methyl 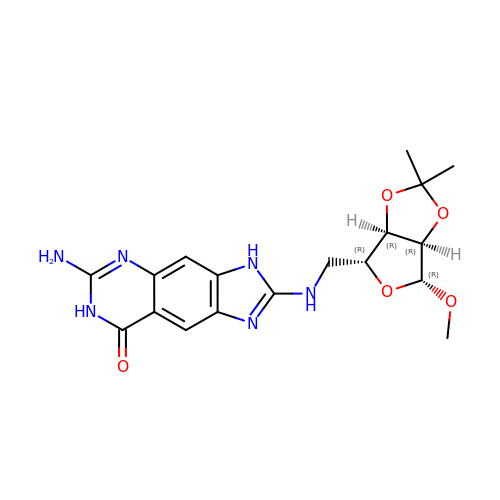5-[(6-amino-8-oxo-7,8-dihydro-3H-imidazo[4,5-g]quinazolin-2-yl)amino]-5-deoxy-2,3-O-(1-methylethylidene)-beta-D-ribofuranoside | C18 H22 N6 O5 | DVNDKLBXQGGFSV-RGCMKSIDSA-N> MTTLLNPYFGEFGGMYVPQILMPALNQLEEAFVSAQKDPEFQAQFADLLKNYAGRPTALTKCQNITAGTRTTLYLKRED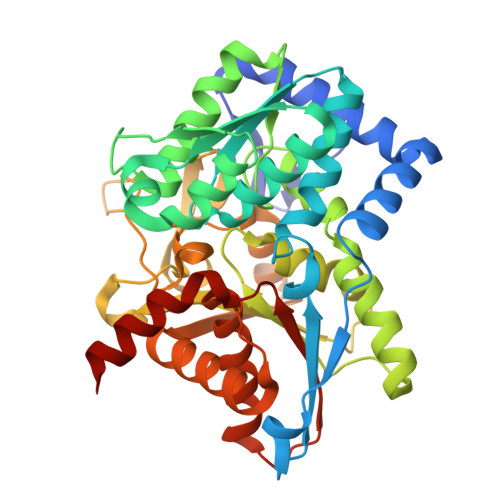LLHGGAHKTNQVLGQALLAKRMGKSEIIAETGAGAHGVASALASALLGLKCRIYMGAKDVERQSPNVFRMRLMGAEVIPVHSGSATLKDACNEALRDWSGSYETAHYMLGTAAGPHPYPTIVREFQRMIGEETKAQILDKEGRLPDAVIACVGGGSNAIGMFADFINDTSVGLIGVEPGGHGIETGEHGAPLKHGRVGIYFGMKAPMMQTADGQIEESYSISAGLDFPSVGPQHAYLNSIGRADYVSITDDEALEAFKTLCRHEGIIPALESSHALAHALKMMREQPEKEQLLVVNLSGRGDKDIFTVHDILKARGEI[(6R)-6-(1H-indazol-4-ylmethyl)-1,4-oxazepan-4-yl]-[1-(4-methoxyphenyl)cyclopentyl]methanone 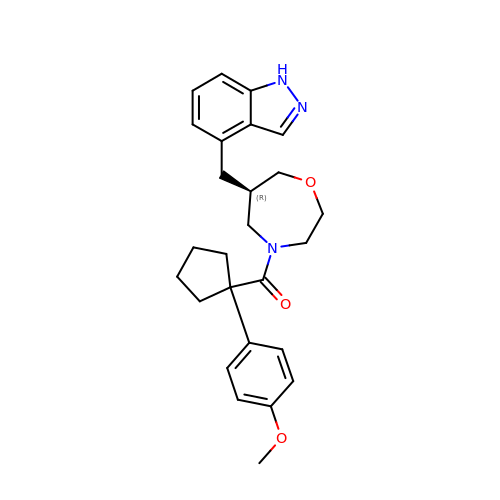| C26 H31 N3 O3 | DUYFMLONWKDSAB-LJQANCHMSA-N> SLLNSRYKLVCYYTNWSWYRPGIGKYSPEDIDPSLCTHIVYGFAVLGNDGLMTAHDTWSDYDNRFYERVVEYKRYGIKVSLALGGWNDSAGDKYSKLVNDPAARAKFVQHAVAFLEKYGFDGLDLDWEYPKCWQVDCSKGPDSDKQGFADLVHELSAVLKPKGLLLSAAVSPNKMVIDAGYDVPVLARLLDWIAVMTYDYHGQWDKKTGHVAPLYYHPDDDTTYFNANYTIHYWMEKGTPASKIVMGMPMYGQSFTIENRGIHGLNIPVSDGGEPGEYTRAKGFLAYYEICDRIRNSGWTVVKDPYQRMGPYAYKGNQWVSFDDVEIIKKKVNF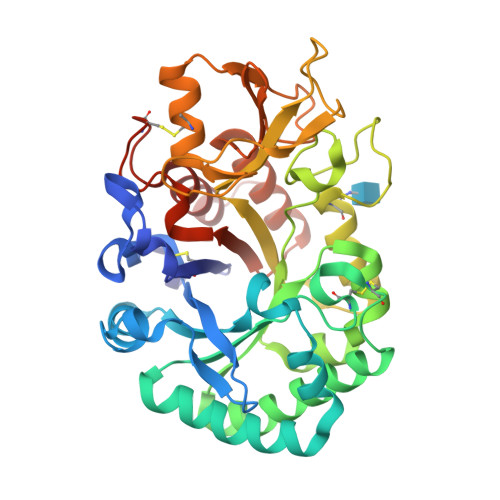IKSLNLGGGMIWALDLDDYRNRCGQGKHPLLNAIKTELLNPKI>MVTARLRPELAGLPVYVPGKTVPGAIKLASNETVFGPLPSVRAAIDRATDTVNRYPDNGCVQLKAALARHLGPDFAPEHVAVGCGSVSLCQQLVQVTASVGDEVVFGWRSFELYPPQVRVAGAIPIQVPLTDHTFDLYAMLATVTDRTRLIFVCNPNNPTSTVVGPDALARFVEAVPAHILIAIDEAYVEYIRDGMRPDSLGLVRAHNNVVVLRTFSKAYGLAGLRIGYAIGHPDVITALDKVYVPFTVSSIGQAAAIASLDAADELLARTDTVVAERARVSAELRAAGFTLPPSQANFVWLPLGSRTQDFVEQAADARIVVRPYGTDGVRVTVAAPEENDAFLRFARRWRSDQKLAAALEH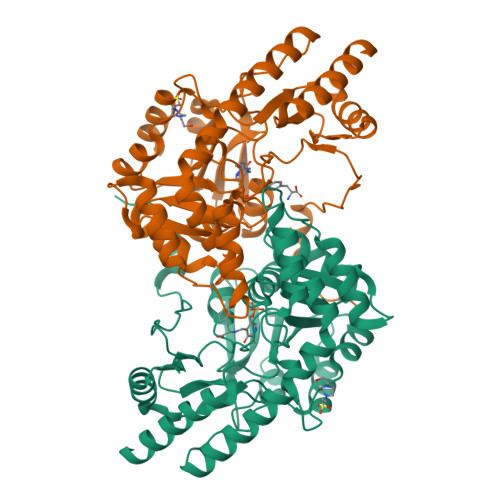HHHHH[4x]>[2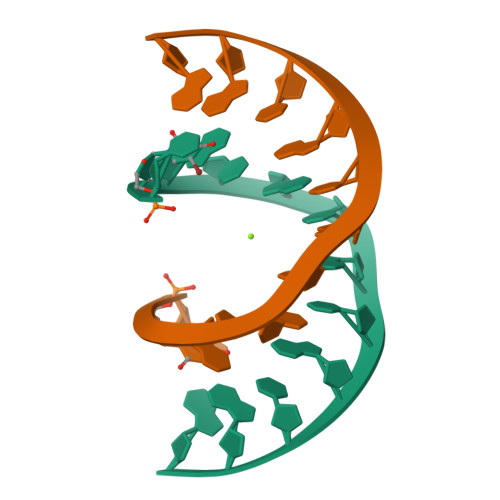x]CUACGCGCGTAG> FFEEMTVYAPVPVPVNGNTHYTSESIERLPTGNGNISDLLRTNPAVRMDSTQSTSLNQGDIRPEKISIHGASPYQNAYLIDGISATNNLNPANESDASSATNISGMSQGYYLDVSLLDNVTLYDSFVPVEFGRFNGGVIDAKIKRFNADDSKVKLGYRTTRSDWLTSHIDENNKSAFNQGSSGSTYYSPDFKKNFYTLSFNQELADNF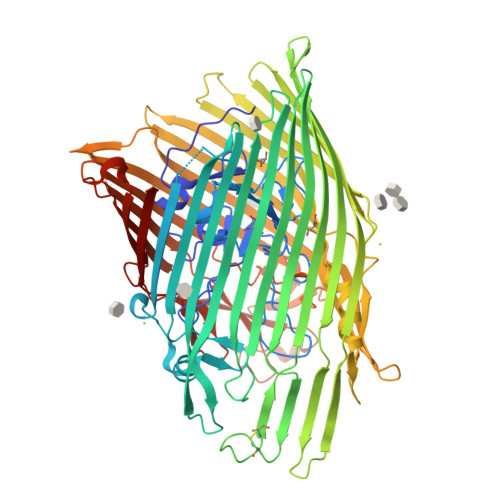GVTAGLSRRQSDITRADYVSNDGIVAGRAQYKNVIDTALSKFTWFASDRFTHDLTLKYTGSSRDYNTSTFPQSDREMGNKSYGLAWDMDTQLAWAKLRTTVGWDHISDYTRHDHDIWYTELSCTYGDITGRCTRGGLGHISQAVDNYTFKTRLDWQKFAVGNVSHQPYFGAEYIYSDAWTERHNQSESYVINAAGKKTNHTIYHKGKGRLGIDNYTLYMADRISWRNVSLMPGVRYDYDNYLSNHNISPRFMTEWDIFANQTSMITAGYNRYYGGNILDMGLRDIRNSWTESVSGNKTLTRYQDLKTPYNDELAMGLQQKIGKNVIARANYVYREAHDQISKSSRTDSATKTTITEYNNDGKTKTHSFSLSFELAEPLHIRQVDINPQIVFSYIKSKGNLSLNNGYEESNTGDNQVVYNGNLVSYDSVPVADFNNPLKISLNMDFTHQPSGLVWANTLAWQEARKARIILGKTNAQYISEYSDYKQYVDEKLDSSLTWDTRLSWTPQFLQQQNLTISADILNVLDSKTAVDTTNTGVATYASGRTFWLDVSMKF> MERYENLFAQLNDRREGAFVPFVTLGDPGIEQSLKIIDTLIDAGADALELGVPFSDPLADGPTIQNANLRAFAAGVTPAQCFEMLALIREKHPTIPIGLLMYANLVFNNGIDAFYARCEQVGVDSVLVADVPVEESAPFRQAALRHNIAPIFICPPNADDDLLRQV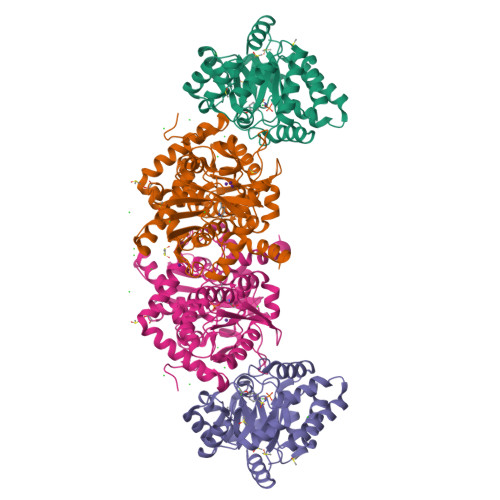ASYGRGYTYLLSRSGVTGAENRGALPLHHLIEKLKEYHAAPALQGFGISSPEQVSAAVRAGAAGAISGSAIVKIIEKNLASPKQMLAELRSFVSAMKAASRA;> TTLLNPYFGEFGGMYVPQILMPALNQLEEAFVSAQKDPEFQAQFADLLKNYAGRPTALTKCQNITAGTRTTLYLKREDLLHGGAHKTNQVLGQALLAKRMGKSEIIAETGAGAHGVASALASALLGLKCRIYMGAKDVERQSPNVFRMRLMGAEVIPVHSGSATLKDACNEALRDWSGSYETAHYMLGTAAGPHPYPTIVREFQRMIGEETKAQILDKEGRLPDAVIACVGGGSNAIGMFADFINDTSVGLIGVEPGGHGIETGEHGAPLKHGRVGIYFGMKAPMMQTADGQIEESYSISAGLDFPSVGPQHAYLNSIGRADYVSITDDEALEAFKTLCRHEGIIPALESSHALAHALKMMREQPEKEQLLVVNLSGRGDKDIFTVHDILKARG>MKKLTIGLIGNPNSGKTTLFNQLTGARQRVGNWAGVTVERKEGQFSTTDHQVTLV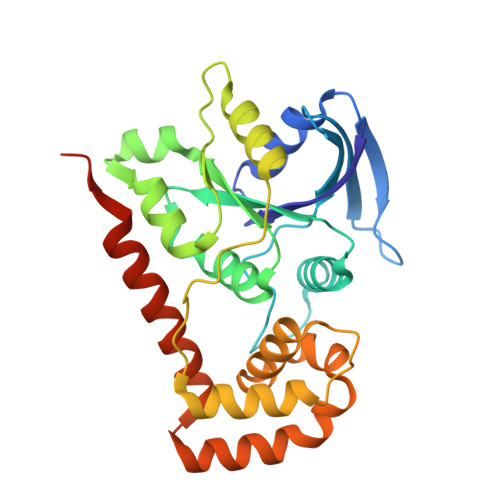DLPGTYSLTTISSQTSLDEQIACHYILSGDADLLINVVDASNLERNLYLTLQLLELGIPCIVALNMLDIAEKQNIRIEIDALSARLGCPVIPLVSTRGRGIEALKLAIDRYKANENVELVHYAQPLLNEADSLAKVMPSDIPLKQRRWLGLQMLEGDIYSRAYAGEASQHLDAALARLRNEMDDPALHIADARYQCIAAICDVVSNTLTAEPSRFTTAV[2x]> MASMSVSTASTEMSVRKIAAHMKSNPNAKVIFMVGAGISTSCGIPDFRSPGTGLYHNLARLKLPYPEAVFDVDFFQSDPLPFYTLAKELYPGNFRPSKFHYLLKLFQDKDVLKRVYTQNIDTLERQAGVKDDLIIEAHGSFAHCHCIGCGKVYPPQVFKSKLAEHPIKDFVKCDVCGELVKPAIVFFGEDLPDSFSETWLNDS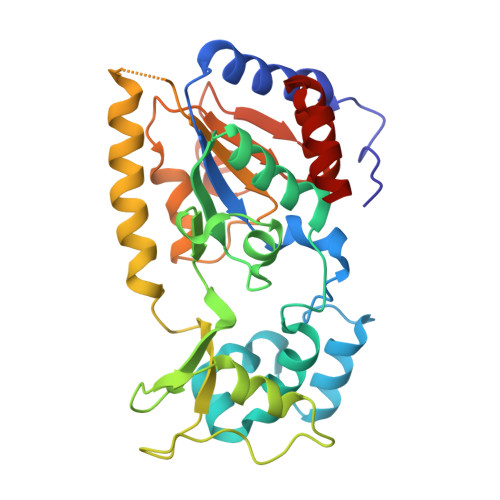EWLREKITTSGKHPQQPLVIVVGTSLAVYPFASLPEEIPRKVKRVLCNLETVGDFKANKRPTDLIVHQYSDEFAEQLVEELGWQEDFEKILTAQ> APLPDTPGAPFPAVANFDRSGPYTVSSQSEGPSCRIYRPRDLGQGGVRHPVILWGNGTGAGPSTYAGLLSHWASHGFVVAAAETSNAGTGREMLACLDYLVRENDTPYGTYSGKLNTGRVGTSGHSQGGGGSIMAGQDTRVRTTAPIQPYTLGLGHDSASQRRQQGPMFLMSGGGDTIAFPYLNAQPVYRRANVPVFWGERRYVSHFEPVGSGGAYRGPSTAWFRFQLMD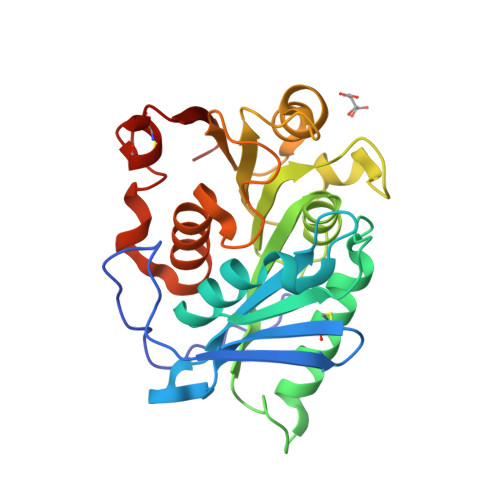DQDARATFYGAQCSLCTSLLWSVERRGL2-azanyl-8-[2-(4-bromophenyl)-2-oxidanylidene-ethyl]sulfanyl-1,9-dihydropurin-6-one | C13 H10 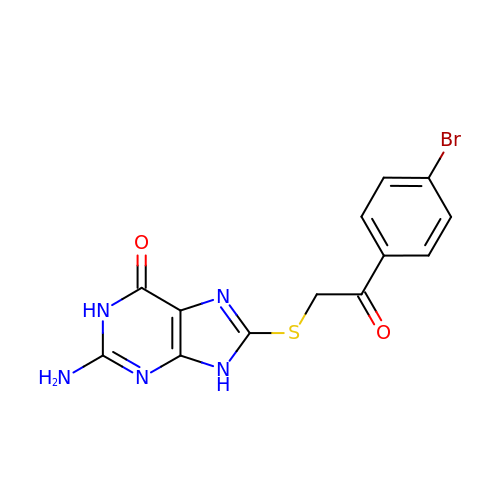Br N5 O2 S | NIDWVLLSHNTXJV-UHFFFAOYSA-N> RLFPPQWICCDIRYLDVSILGKFAVVMADPPWDIHMELPYGTLTDDEMRRLNIPVLQDDGFLFLWVTGRAMELGRECLNLWGYERVDEIIWVKTNQLQRIIRTGRTGHWLNHGKEHCLVGVKGNPQGFNQGLDCDVIVAE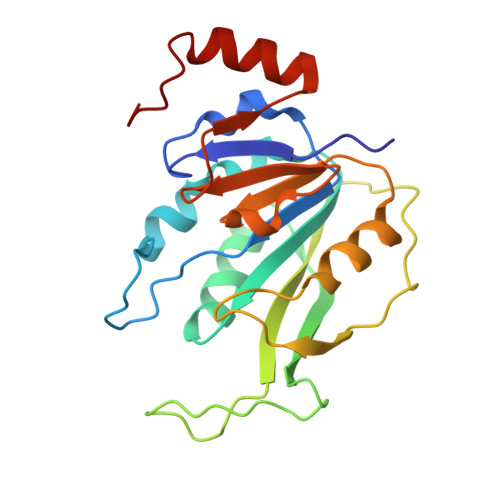VRSTSHKPDEIYGMIERLSPGTRKIELFGRPHNVQPNWITLGNQLDGIHLLDPDVVARFKQRYPDGIISKP>MAIITPALISALKTSFQKHFQDALATAPSTYLQVATVIPSTTASNTYGWLGQFPKLREWIGQRVIKDMAAQGYQITNKLFESTVGVKRTDIEDDNLGVYGPLMQEMGRAAGAHPDELVFALLKAGNANLCYDGQNFFDTDHPVYPNVDGTGTATTVSNLFAPAADPGAAWYLLDTSRSLKPLIYQERMKPSFTSMTKEDDEQVFMADEYRYGVRSRCNVGFGFWQLAAMSTEELNQVNFEKVYDAMRNQKADGGRPLDIRPNLLVVPTTLRSKAKEVVGVQRLANGADNPNFELVQVLDTAWLN[7x]

Bacteriophage Casadabanvirus JBD30, from the order Caudoviricetes, is a temperate phage that infects the bacterium Pseudomonas aeruginosa. The virion of bacteriophage JBD30 is composed of an icosahedral capsid, long flexible non-contractile tail, and a baseplate. Using its baseplate, JBD30 attaches to Pseudomonas aeruginosa via the bacterial type IV pilus, whose subsequent retraction brings the phage to the bacterial cell surface.

Here we present the structures of the virion and empty particle of siphophage JBD30 resolved using cryo-electron microscopy. The icosahedral capsid of bacteriophage JBD30 is built from 415 copies of major capsid proteins organised in a T7 laevo lattice. The capsid of JBD30 is formed by pentamers and hexamers of major capsid proteins. Unlike in phage HK97, there are no covalent bonds linking the capsid proteins to each other. The positioning of annular loops extending from the axial domains leaves openings in the centre of hexamers (7 Å radius) and pentamers (6 Å radius). These pores were suggested to serve for water and ion passage during genome packaging and ejection, and putative scaffold protein release during capsid maturation. The empty JBD30 particle remains associated with the cell wall.> MLQEQSELMSTVMNNTPTTVAALAAVAAASETNGKLGSEEQPEITIPKPRSSAQLEQLLYRYRAIQNHPKENKLEIKAIEDTFRNISRDQDIYETKLDTLRKSIDKGFQYDEDLLNKHLVALQLLEKDTDVPDYFLDLPDTKNDNTTAIEVDYSEKKPIKISADFNAKAKSLGLESKFSNATKTALGDPDTEIRISARISNRINELERLPANLGTYSLDDCLEFITKDDLSSRMDTFKIKALVELKSLKLLTKQKSIRQKLINNVASQAHHNIPYLRDSPFTAAAQRSVQIRSKVIVPQTVRLAEELERQQLLEKRKKERNLHLQKINSIIDFIKERQSEQWSR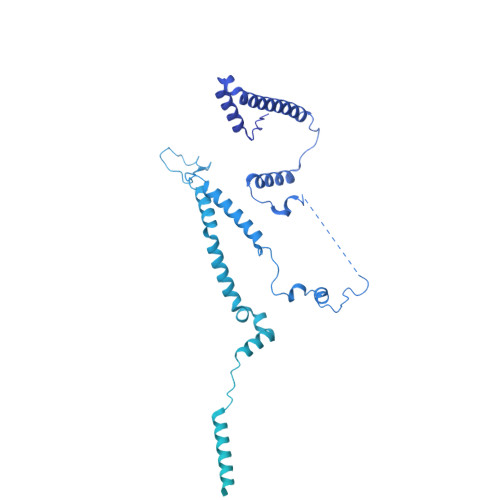QERCFQFGRLGASLHNQMEKDEQKRIERTAKQRLAALKSNDEEAYLKLLDQTKDTRITQLLRQTNSFLDSLSEAVRAQQNEAKILHGEEVQPITDEEREKTDYYEVAHRIKEKIDKQPSILVGGTLKEYQLRGLEWMVSLYNNHLNGILADEMGLGKTIQSISLITYLYEVKKDIGPFLVIVPLSTITNWTLEFEKWAPSLNTIIYKGTPNQRHSLQHQIRVGNFDVLLTTYEYIIKDKSLLSKHDWAHMIIDEGHRMKNAQSKLSFTISHYYRTRNRLILTGTPLQNNLPELWALLNFVLPKIFNSAKTFEDWFNTPFANTGTQEKLELTEEETLLIIRRLHKVLRPFLLRRLKKEVEKDLPDKVEKVIKCKLSGLQQQLYQQMLKHNALFVGAGTEGATKGGIKGLNNKIMQLRKICNHPFVFDEVEGVVNPSRGNSDLLFRVAGKFELLDRVLPKFKASGHRVLMFFQMTQVMDIMEDFLRMKDLKYMRLDGSTKTEERTEMLNAFNAPDSDYFCFLLSTRAGGLGLNLQTADTVIIFDTDWNPHQDLQAQDRAHRIGQKNEVRILRLITTDSVEEVILERAMQKLDIDGKVIQAGKFDNKSTAEEQEAFLRRLIESETNRDDDDKAELDDDELNDTLARSADEKILFDKIDKERMNQERADAKAQGLRVPPPRLIQLDELPKVFREDIEEHFKKEDSEPLGRIRQKKRVYYDDGLTEEQFLEAVEDDNMSLEDAIKKRREARERRRLRQNGTKENEIETLENTPEASETSLIENNSFTAAVDEETNADKETTASRSKRRSSRKKRTISIVTAEDKENTQEESTSQENGGAKVEEEVKSSSVEIINGSESKKKKPKLTVKIKLNKTTVLENNDGKRAEEKPESKSPAKKTAAKKTKTKSKSLGIFPTVEKLVEEMREQLDEVDSHPRTSIFEKLPSKRDYPDYFKVIEKPMAIDIILKNCKNGTYKTLEEVRQALQTMFENARFYNEEGSWVYVDADKLNEFTDEWFKEHSS>MRTPYCVADYLLDRLTDCGADHLFGVPGDYNLQFLDHVIDSPDICWVGCANELNASYAADGYARCKGFAALLTTFGVGELSAMNGIAGSYAEHVPVLHIVGAPGTAAQQRGELLHHTLGDGEFRHFYHMSEPITVAQAVLTEQNACYEIDRVLTTMLRERRPGYLMLPADVAKKAATPPVNALTHKQAHADSACLKAFRDAAENKLAMSKRTALLADFLVLRHGLKHALQKWVKEVPMAHATMLMGKGIFDERQAGFYGTYSGSASTGAVKEAIEGADTVLCVGTRFTDTLTAGFTHQLTPAQTIEVQPHAARVGDVWFTGIPMNQAIETLVELCKQHVHAGLMSSSSGAIPFPQPDGSLTQENFWRTLQTFIRPGDIILADQGTSAFGAIDLRLPADVNFIVQPLWGSIGYTLAAAFGAQTACPNRRVIVLTGDGAAQLTIQELGSMLRDKQHPIILVLNNEGY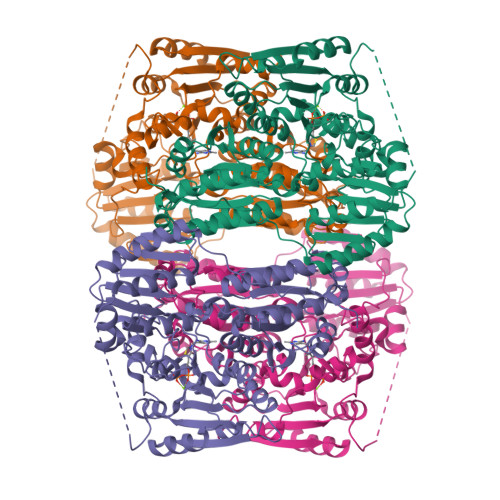TVERAIHGAEQRYNDIALWNWTHIPQALSLDPQSECWRVSEAEQLADVLEKVAHHERLSLIEVMLPKADIPPLLGALTKALEACNNA[4x]> MGEEAELAYLLGELAYKLGEYRIAIRAYRIALKRDPNNAEAWYNLGNAYYKQGDYDEAIEYYQKALELDPNNAEAWYNLGNAYYKQGDYDEAIEYYEKALELDPENLEALQNLLNAMDKQG;> MIEEVVAEMIDILAESSKKSIEELARAADNKTTEKAVAEAIEEIARLATAAIQLIEALAKNLASEEFMARAISAIAELAKKAIEAIYRLADNHTTDTFMARAIAAIANLAVTAILAIAALASNHTTEEFM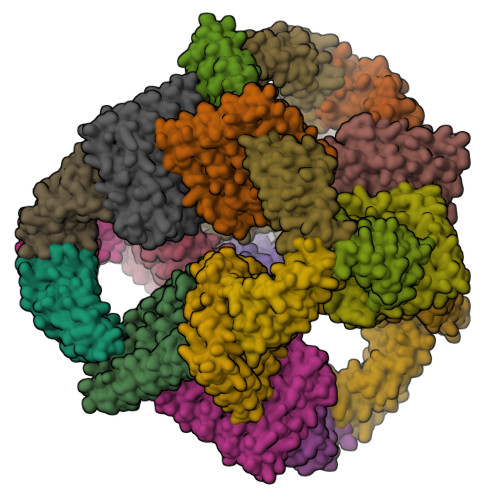ARAISAIAELAKKAIEAIYRLADNHTTDKFMAAAIEAIALLATLAILAIALLASNHTTEKFMARAIMAIAILAAKAIEAIYRLADNHTSPTYIEKAIEAIEKIARKAIKAIEMLAKNITTEEYKEKAKKIIDIIRKLAKMAIKKLEDNRTLEHHHHHH>[2x]MSENLKDEILEKYIPKTKKTR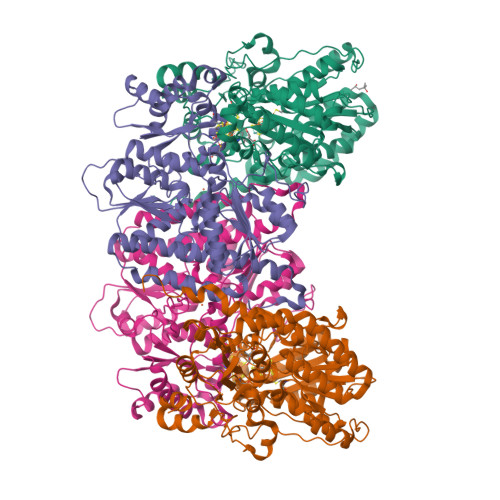SGHIVIKTEETPNPEIVANTRTVPGIITARGCAYAGCKGVVMGPIKDMVHITHGPIGCSFYTWGGRRFKSKPENGTGLNFNEYVFSTDMQESDIVFGGVNKLKDAIHEAYEMFHPAAIGVYATCPVGLIGDDILAVAATASKEIGIPVHAFSCEGYKGVSQSAGHHIANNTVMTDIIGKGNKEQKKYSINVLGEYNIGGDAWEMDRVLEKIGYHVNATLTGDATYEKVQNADKADLNLVQCHRSINYIAEMMETKYGIPWIKCNFIGVDGIVETLRDMAKCFDDPELTKRTEEVIAEEIAAIQDDLDYFKEKLQGKTACLYVGGSRSHTYMNMLKSFGVDSLVAGFEFAHRDDYEGREVIPTIKIDADSKNIPEITVTPDEQKYRVVIPEDKVEELKKAGVPLSSYGGMMKEMHDGTILIDDMNHHDMEVVLEKLKPDMFFAGIKEKFVIQKGGVLSKQLHSYDYNGPYAGFRGVVNFGHELVNGIYTPAWKMITPPWKKASSESKVVVGGEA;>MLDATPKEIVERKALRINPAKTCQPVGAMYAALGIHNCLPHSHGSQGCCSYHRTVLSRHFKEPAMASTSSFTEGASVFGGGSNIKTAVKNIFSLYNPDIIAVHTTCLSETLGDDLPTYISQMEDAGSIPEGKLVIHTNTPSYVGSHVTGFANMVQGIVNYLSENTGAKNGKINVIPGFVGPADMREIKRLFEAMDIPYIMFPDTSGVLDGPTTGEYKMYPEGGTKIEDLKDTGNSDLTLSLGSYASDLGAKTLEKKCKVPFKTLRTPIGVSATDEFIMALSEATGKEVPASIEEERGQLIDLMIDAQQYLQGKKVALLGDPDEIIALSKFIIELGAIPKYVVTGTPGMKFQKEIDAMLAEAGIEGSKVKVEGDFFDVHQWIKNEGVDLLISNTYGKFIAREENIPFVRFGFPIMDRYGHYYNPKVGYKGAIRLVEEITNVILDKIERECTEEDFEVVR[2x]(E)-[7-azanyl-10-[2-carboxy-5-[2-[2-(6-chloranylhexoxy)ethoxy]ethylcarbamoyl]phenyl]-5,5-dimethyl-benzo[b][1]benzosilin-3-ylidene]-methyl-azanium 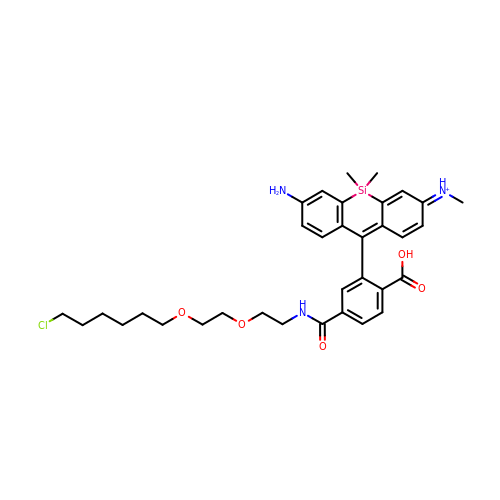| C34 H43 Cl N3 O5 Si | HVINIPVEAAMTAU-AUGOTPMTSA-O CYP124 (Rv2266, CYP124A1) has previously assigned activity towards methyl-branched lipids of isoprenoid origin, while CYP125 (Rv3545c, CYP125A1) and CYP142 (Rv3518c, CYP142A1) are involved in the cholesterol catabolism. Multiple substrates have been previously identified for CYP124, including cholesterol, vitamin D, their derivatives, and methyl-branched lipids. Although its physiological function and, therefore, a natural substrate is not yet confirmed, there is a common pattern among all the substrates—a methyl-branched tail, tightly positioned for ω-hydroxylation in the distal site. SQ109 belongs to the 1,2-ethylenediamine class of anti-TB drugs, consisting of adamantane head and geranyl tail, proposed to disrupt the synthesis of the complex Mtb cell wall.

To determine the binding mode and the hydroxylation position, we co-crystallized SQ109 with CYP124. A 1.25 Å crystal structure of the CYP124–SQ109 complex reveals two close conformations of SQ109, confirming the formation of a ω-terminal hydroxy product. The 2mFo−DFc composite omit map unambiguously shows SQ109 density in two conformations, which differ only in the ethylenediamine-adamantane part. At the same time, geranyl tails in both conformations are positioned above Fe in the typical geometry for ω- hydroxylation. Distances between the heme iron and the carbon atoms of the branched methyl groups are 4.0 Å and 6.1 Å, which favorites the hydroxylation of the ω-methyl group in the trans position. Thus, CYP124 catalyzes the regio- and stereo-selective hydroxylation of SQ109. The geranyl tail is tightly enclosed in the narrow tunnel with a broadening to accommodate ω-5 methyl branching position (methyl at C3 of SQ109). In contrast, adamantane and ethylenediamine are positioned more freely in a wide cavity in the upper part of the binding pocket. The interactions of SQ109 are mostly hydrophobic (L60, F63, T96, and F212 interact with the adamantane; F107, I111, L198, L263, V266, A267, F416, and I417 fix the aliphatic chain), while in the predominant conformation (A), the drug could potentially form a weak hydrogen bond with HOH879. The absence of stabilizing H-bonds might result in the emergence of two conformations of the adamantane group.

> MHHHHHHMGLNTAIATRVNGTPPPEVPIADIELGSLDFWALDDDVRDGAFATLRREAPISFWPTIELPGFVAGNGHWALTKYDDVFYASRHPDIFSSYPNITINDQTPELAEYFGSMIVLDDPRHQRLRSIVSRAFTPKVVARIEAAVRDRAHRLVSSMIANNPDRQADLVSELAGPLPLQIICDMMGIPKADHQRIFHWTNVILGFGDPDLATDFDEFMQVSADIGAYATALAEDRRVNHHDDLTSSLVEAEVDGERLSSREIASFFILLVVAGNETTRNAITHGVLALSRYPEQRDRWWSDFDGLAPTAVEEIVRWASPVVYMRRTLTQDIELRGTKMAAGDKVSLWYCSANRDESKFADPWTFDLARNPNPHLGFGGGGAHFCLGANLARREIRVAFDELRRQMPDVVATEEPARLLSQFIHGIKTLPVTWS(2~{S})-2-azanyl-1-[(1~{S},3~{S},5~{S})-3-(iminomethyl)-2-azabicyclo[3.1.0]hexan-2-yl]-2-[(5~{R},7~{S})-3-oxidanyl-1-adamantyl]ethanone 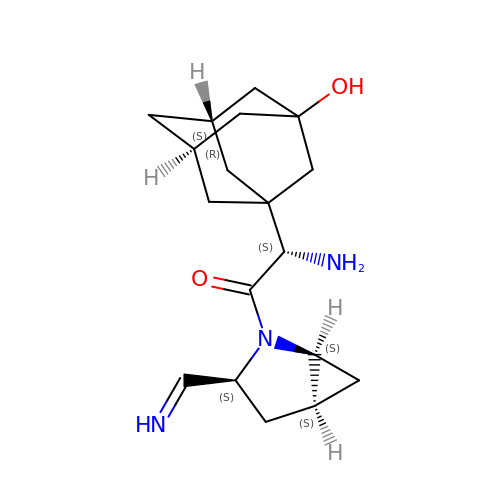| C18 H27 N3 O2 | KMSQNYQXZPWGMJ-YQBUGCKMSA-N> QTIQSIPQKGFFGHPRGLGVLFFVEFWERFSYYGMRAMLIFYMYFAIHQNGLGIDKTTAMSIMSVYGALIYMSSIPGAWIADRITGTRGATLLGAVLIIIGHICLSLPFALFGLFSSMFFIIIGSGLMKPNISNIVGRLYPE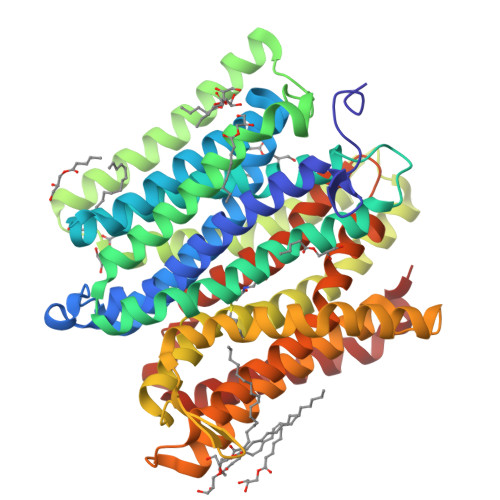NDTRIDAGFVIFYMSVNLGALISPIILQHFVDIRNFHGGFLLAAIGMALGLVWYLLFNRKNLGSVGMAPTNPLSKEEKRKYGMIIGIIVAIVIVVLLVTYYTHTLSFDLISNTVLVLGVALPIIYFTTMLRSKDVTDGERSRVKAFIPLFILGMLFWSIQEQGSNVLNIYGLERSDMQLNLFGWTTRFGEALFQSINPLFILLFAPVISMIWLKMGKKQPSLAIKFSIGTLLAGLSYILIGLVGLGYGHTQFSVNWVILSYVICVIGELCLSPTGNSAAVKLAPKAFNAQMMSVWLLTNASAQAINGTLVKLIKPLGQTNYFIFLGTVAIVITLIILVFSPKITK The ComABCDE pathway is the quorum-sensing system in some species of Streptococcus, such as S. mutans and S. pneumoniae, in which autoinducer peptides are processed from the precursor ComC and concomitantly exported to the extracellular space by ComA and ComB6, 7. PEP is a highly specific peptidase belonging to a cysteine protease family. We believe that PEP of ComA is a more suitable target for inhibitor development for the following reasons: First, PEP catalyzes the initial step of the quorum-sensing system of Streptococcus. In this study, we focused on PEP as the target of potential inhibitors of the Streptococcus quorum-sensing pathway, established a reliable high-throughput screening system using a synthetic substrate for PEP, and successfully obtained a compound that was found to allosterically inhibit PEP and suppress the quorum-sensing pathway, which eventually led to attenuated biofilm formation.

To address this idea, we tried to resolve the structure of MuPEP1 complexed with Compound 1 by soaking and co-crystallization methods under various conditions, but the diffraction data revealed no bound compound molecule. In the crystal structure of the original MuPEP1, this pocket is occupied by residues from the adjacent protein molecule, which would explain why the complex structure could not be obtained. Therefore, we prepared another form of MuPEP1 with the four N-terminal residues truncated (tMuPEP1), a form that was found to be crystallized in a different space group from that of MuPEP1. The side chain of Arg66 occupies the vacant space of this binding pocket in free tMuPEP1, whereas it is rotated away to avoid steric hindrance with Compound 2 in the tMuPEP1-Compound 2 complex. There are no other significant differences in either the overall structure or the catalytic triad residues between the free and complex structures of tMuPEP1.

>[2x]MYKLVPQIDTRDCGPAVLASVAKHYGSNYSIAYLRELSKTNKQGTTALGIVEAAKKLGFETRSIKADMTLFDYNDLTYPFIVHVIKGKRLQHYYVVYGSQNNQLIIGDPDPSVKVTRMSKERFQSEWTGLAIFLAPQPNYKPHKGEHHHHHH>HHHHHHHHGGLVPRGSHGGSMTDRLKGKVAIVTGGTLGIGLAIADKFVEEGAKVVITGRHADVGEKAAKSIGGTDVIRFVQHDASDEAGWTKLFDTTEEAFGPVTTVVNNAGIAVSKSVEDTTTEEWRKLLSVNLDGVFFGTRLGIQRMKNKGLGASIINMSSIEGFVGDPTLGAYNASKGAVRIMSKSAALDCALKDYDVRVNTVHPGYIKTPLVDDLEGAEEMMSQRTKTPMGHIGEPNDIAWICVYLASDESKFA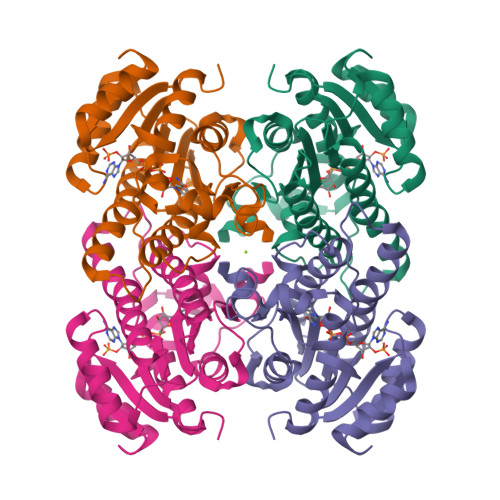TGAEFVVDGGYTAQ[2x]> LEEGSYVRIKRGIYKGDLAMVDQISENNLEVMLKIVPRLDYGKFDEIDPTTQQRKSRRPTFAHRAPPQLFNPTMALRLDQANLYKRDDRHFTYKNEDYIDGYLYKSFRIQHVETKN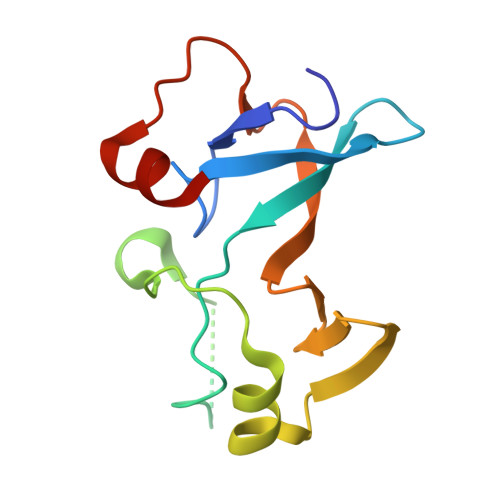IQPTVEELARFGSK> APVRSLNCTLRDSQQKSLVMSGPYELKALHLQGQDMEQQVVFSMSFVQGEESNDKIPVALGLKEKNLYLSAVLKDDKPTLQLESVDPKNYPKKKMEKRFVFNKIEINNKLEF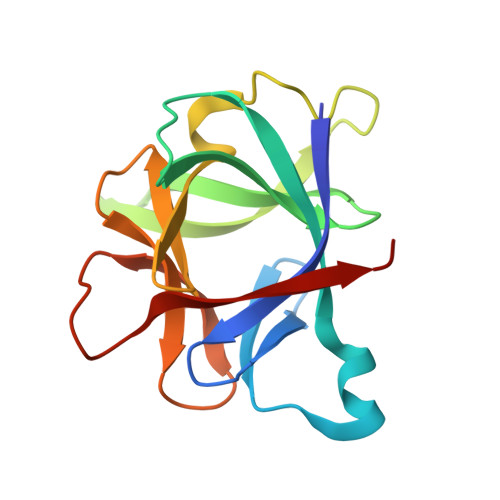ESAQFPNWYISTSQAENMPVFLGGTKGGQDITDFTMQFVSS> MNVIAILNHMGVYFKEEPIRELHRALERLNFQIVYPNDRDDLLKLIENNARLCGVIFDWDKYNLELCEEISKMNENLPLYAFANTYSTLDVSLNDLRLQISFFEYALGAAEDIANKIKQTTDEYINTILPPLTKALFKYVREGKYTFCTPGHMGGTAFQKSPVGSLFYDFFGPNTMKSDISISVSELGSLLDHSGPHKEAEQYIARVFNADRSYMVTNGTSTANKIVGMYSAPAGSTILIDRNCHKSLTHLMMMSDVTPIYFRPTRNAYGILGGIPQSEFQHATIAKRVKETPNATWPVHAVITNSTYDGLLYNTDFIKKTLDVKSIHFDSAWVPYTNFSPIYEGKCGMSGGRVEGKVIYETQSTHKLLAAFSQASMIHVKGDVNEETFNEAYMMHTTTSPHYGIVASTETAAAMMKGNAGKRLINGSIERAIKFRKEIKRLRTESDGWFFDVWQPDHIDTTECWPLRSDSTWHGFKNIDNEHMYLDPIKVTLLTPGMEKDGTMSDFGIPASIVAKYLDEHGIVVEKTGPYNLLFLFSIGIDKTKALSLLRALTDFKRAFDLNLRVKNMLPSLYREDPEFYENMRIQELAQNIHKLIVHHNLPDLMYRAFEVLPTMVMTPYAAFQKELHGMTEEVYLDEMVGRINANMILPYPPGVPLVMPGEMITEESRPVLEFLQMLCEIGAHYPGFETDIHGAYRQADGRYTVKVLKEESKK;> GHMQQSDKTALTVIRLGGIFSRRQQYQLPVNVTASTLTLLLQK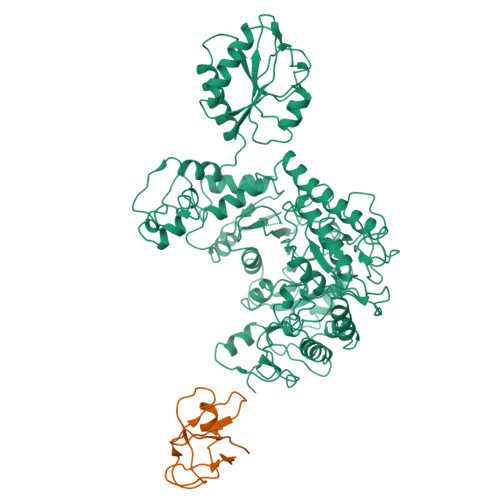PLKLHDMEVVHISFERSALEQWLSKGGEIRGKLNGIGFAQKLNLEVDSAQHLVVRDVSLQGSTLALPGSSAE>[2x]MASIPSAAPSWRKMQIPRPLQRLFDYFPLRIYEPNELPERSQQLTSGDLPTLYVFSTDSDARLGLPSFNPGCLKWQTLLRLANLDFRILPSTNHSSPTG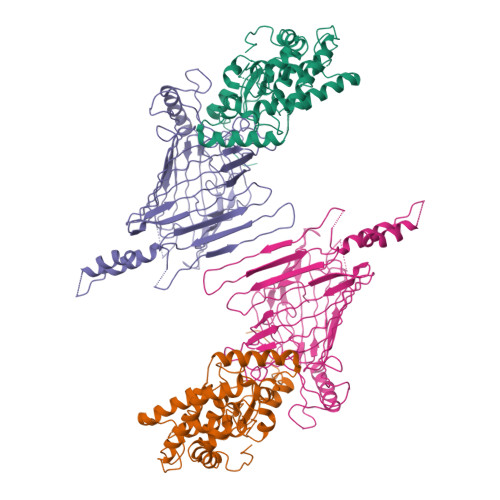SLPFLLPPRTSPTASPAPIPASGLLSFARKNPWRPGKAADLDLGHLDADLPPRAQAYLALITHSLRNAWLCALYLDPTHDALLRRLYVDPASSSRAVRAALLHQLRRAAAEQVATASSGGGKIVSLAPVDSADGIDEEAVYRSARDALDALASLLRESETAWFGTERPGSFDAALFSYTHLMVEYMSEEEDTESAKGRVSLGRMVKEAGNGELAEHRERMLGVAWPEWDGYRR;>[2x]MASSLGFGGSNAVDKVNATTTPGTVATPNSGPTKMLDEHILTPASISTLEVHGATNTRRSLLDQIFKPVLEDTAAAGTTLGQVLDRVGAATKKLARFDIFKEEGFGVFLSEAAPPQSAPPTDRTDLDISIRVKEKSRLVFSAGTDFGNAEGSAYTNAVVRNIFGGAETLTVNASTGTRTRSAYNATFSTPINGNPDLRLSVEALRSATQKPWASHEEHLTGANLRLAWLTEKGDTHALAYSSVWRQLTGLAPTASPTVRADAGDSLKSSLTHTFTRDRRDNPMLPQSGYLFRSVSELAGWGPLNGDVSFAKTEVEASGALPVAIPGLAGKSGVSVGGGLRLGVLYPLPLGYSLTGAAQPSRINDRFQLGGPNDVRGFKIGGLGPHDGVDAVGGDVFAAGSVNALLPLPRTGPDSPLRLQLYANAGRLVALNSKGTDKEGKEGLAMDSAAVFKGVKSAVGKLTNGIPSLAAGVGLVYAHPVARFELNFSLPLVLRRGEEGRKGLQVGVGISFL MDHAR reduces the monodehydroascorbate (MDHA) radical to AsA at the expense of an NAD(P)H molecule, with NADH being the preferred donor. We report, for the first time, the crystal structure of MDHAR of O. sativa L. japonica (OsMDHAR) to understand its detailed mechanism. Structural comparison of OsMDHAR to other proteins, using the DALI server, indicated that it has the same fold as that of putidaredoxin reductase (Pdr), biphenyl dioxygenase (BphA4)18 and rubredoxin reductase (RdxR). All these proteins consist of three domains: an NAD(P)-binding domain, an FAD-binding domain, and a C-terminal domain, as shown in Figs 1 and 2.

For structural confirmation of binding of the enzyme to an AsA analogue, we co-crystallized OsMDHAR bound to NADH and isoascorbic acid (ISD), as D-erythroascorbic acid is not commercially available. We observed an interpretable electron density map, suitable for ISD fitting. Superimposed structures of OsMDHAR-AsA and OsMDHAR-ISD complexes showed distinct binding conformations for both substrate ligands. In detail, ISD did not fit perfectly into the binding site of AsA. The binding site of ISD had more exposed surface area. In addition, we observed clear electron density for the di-hydroxyfuranone part of ISD, but not its di-hydroxyethyl part. This suggests that ISD may bind more loosely to the enzyme than AsA. Nevertheless, ISD is hydrogen bonded to the conserved Arg320, which is within an accessible distance for electron transfer from the Tyr349 residue. The Arg320 residue forms hydrogen bonds with both AsA and ISD in the complex structures. Given the structural and functional analysis, we conclude that the binding site of OsMDHAR may be able to accommodate variable substrate compositions including MDHA.

>HHHHHHASENLYFQGAMASEKHFKYVILGGGVAAGYAAREFAKQGVKPGELAIISKEAVAPYERPALSKGYLFPQNAARLPGFHVCVGSGGERLLPEWYSEKGIELILSTEIVKADLASKTLTSAVGATFTYEILIIATGSSVIKLSDFGTQGADSNNILYLREVDDADKLVAAIQAKKGGKAVIVGGGYIGLELSAALKINDFDVTMVFPEPWCMPRLFTADIAAFYESYYTNKGVKIVKGTVAVGFDADANGDVTAVNLKNGSVLEADIVVVGVGGRPLTTLFKGQVAEEKGGIKTDAFFETSVPGVYAVGDVATFPMKMYNELRRVEHVDHARKSAEQAVKAIKGKESGESVVEYDYLPYFFSRSFDLGWQFYGDNVGDTILFGDSDPTSAKPKFGSYWIKDGKVLGAFLEGGSPDENKAIAKVAKTQPPVANIEELKKEGLQFASKI[2x]>MTHSLKALFALLFLYTAAVNAGVIGIFNALPPPNTKPINGESPLYQCDILDKQLVEIKEVNLDPNPPVRGENLTISANGEVFETIEEGAYIDVEVRLGYIRLLSQTFDLCETLEDNDIEGLSCPIEPGEYNIKKIVEI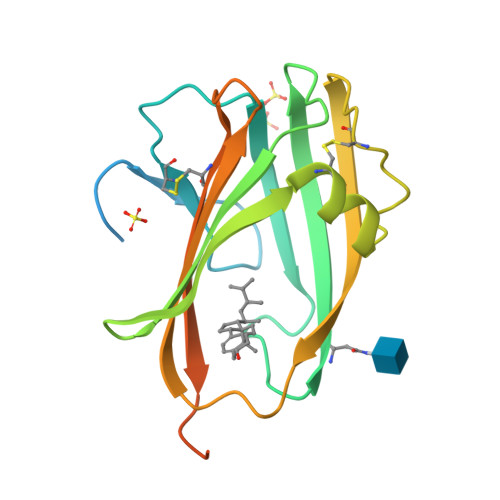PGEVPPGKYVVVARAYTEKDDLITCLTGEVIFPPRLVPRGSGGGGSGGGGSGGHHHHHHHHHH[9x]The earliest discovered selective autophagy pathway in Saccharomyces (S.) cerevisiae is the cytoplasm‐to‐vacuole targeting (Cvt) pathway, through which hydrolytic enzymes are sequestered into double‐membrane vesicles, termed Cvt vesicles, and transported to the vacuole 8, 9. The best‐characterized cargo component of the Cvt vesicle is the vacuolar aminopeptidase I (Ape1) 16. Ape1 is synthesized in the cytosol as a 55‐kDa zymogen that includes an N‐terminal propeptide (hereafter referred to as prApe1), which oligomerizes into a dodecamer 17, 18 and further assembles into larger aggregates in a propeptide‐dependent manner 19. In addition to prApe1, Atg19 also binds another cargo hydrolase α‐mannosidase 1 (Ams1) 25, 26 via a site distinct from the prApe1 binding site, thus forming the Cvt complex.

In order to further improve the resolution of the mApe1 EM structure, we used an Ape1 homolog of 40% sequence identity from the thermophilic filamentous fungus Chaetomium (C.) thermophilum (ct‐mApe1) 30, to exploit increased stability of dodecameric species when compared with sc‐mApe1 (Fig EV1). Moreover, we determined the crystal structure of ct‐mApe1 organized in dodecamers at 2.8 Å resolution. In the crystal, ct‐mApe1 is present as dodecamers, which are formed by two asymmetric units each containing six ct‐mApe1 molecules. Cartoon representation of ct‐mApe1 structure including the catalytic domain (cyan) and the ancillary domain (magenta). The binuclear Zn2+ center bridged by the bidentate ligand Asp259 of the active site is located at the top of the catalytic domain. A conserved histidine residue (His163) belonging to the neighboring subunit protrudes into the active site. Dimerization via the ancillary domains forms the edges of the tetrahedron (left). A book page view along one of the body diagonals reveals the catalytic sites (Zn2+, yellow spheres) that are buried inside the hollow tetrahedral core (right). The amino termini (orange circles) are located on the facets of the tetrahedron. The superposition shows a close structural overlap of the dodecamer assemblies except for a noticeable difference in the active site that is well defined in our structure due to the presence of the cofactor zinc, but disordered in the sc‐mApe1 crystal (Fig EV2G).

>[6x]MTRLTPDVLRMRSSQLSLRSLAMEQPQQRTAAPPTIDEAPTVPLEAKDLRPEHFTQPYLDFMTHNPTVFHVVDYCKQKLLKAGYVELPARDSWTGKLVPGGKYFTTRNGSSIIAFTVGQAYKPGNGIAMIAGHIDALTARLKPTSVKPTKEGYVQLGVAQYAGALNETWWDRDLSVGGRVIVKDPKTGKTTVKLVKVDWPVARIPTLAPHFGIGMTGHGNRETEMVPVIGIDNSDLLGEKAESEKPVGKPGSFASTQPPKLVKLILSQLGLSDPDSILNWELELFDAQPATVGGLDKEFIFAGRIDDKLCSWAAFMALLHAKRAPTDGVIKLVALFDDEEIGSLLRQGARGNFLPITIERILESFCSSNSVPFGPGILGQTYARSFLVSSDVTHAAHPNFTQTNLPGHSPRLNVGVALCVDASAHMTTDSVSMAILDRIAELSGCVNQRHMIRNDSRSGGTVGPMLSAAMGVKAADVGIPQLSMHSIRAMTGSLDPGLGVKFYKGFLDFWEEVDLEWSH>GASGDGAGASRQRKLEALIRDPRSPINVESLLDGLNSLVLDLDFPALRKNKNIDNFLNRYEKIVKKIRGLQMKAEDYDVVKVIGRGAFGEVQLVRHKASQKVYAMKLLSKFEMIKRSDSAFFWEERDIMAFANSPWVVQLFCAFQDDKYLYMVMEYMPGGDLVNLMSNYDVPEKWAKFYTAEVVLALDAIHSMGLIHRDVKPDNMLLDKHGHLKLADFGTCMKMDETGMVHCDTAVGTPDYISPEVLKSQGGDGYYGRECDWWSVGVFLFEMLVGDTPFYADSLVGTYSKIMDHKNSLCFPEDAEISKHAKNLICAFLTDREVRLGRNGVEEIKQHPFFKNDQWNWDNIRETAAPVVPELSSDIDSSNF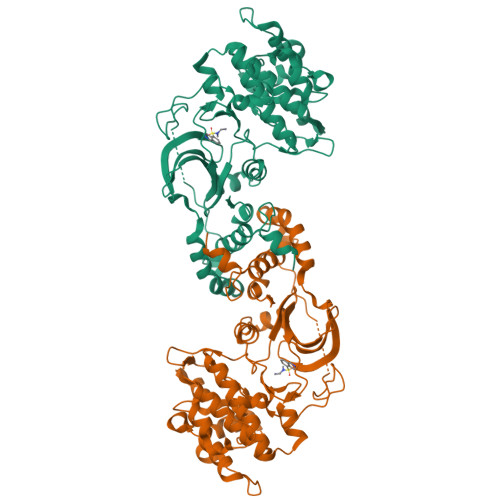DDIEDDKGDVETFPIPKAFVGNQLPFIGFTYYR[2x]> MLSKTILDKLNHQVNFEAASAHLYLQMSAWLLTQSLDSTAAFFRAHAEEEKAHMMKLFDYINETGSLALIGEVATPAPEWKSHIELLEAAYNHELAITQSINDLVDTALREKDYSTFQFLQWYVAEQHEEEYLFSSMLHKARII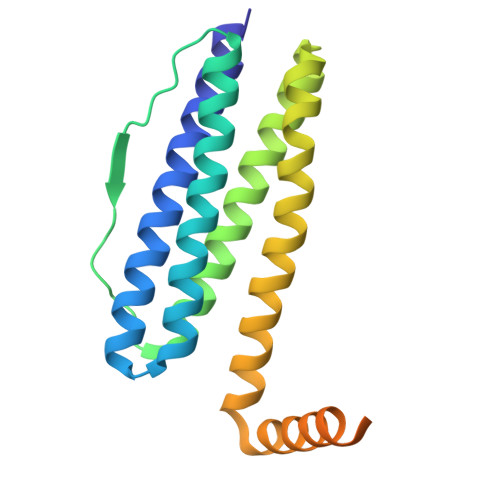NTMDGRALFRFDEEVRKSVLHHEHHQQKPMFLQVGPAPKHHDGHDGLHAHQHSSHWSGH>MPFTYSIEATRNLATTERCIQDIRNAPVRNRSTQFQLAQQNMLAYTFGEVIPGFASAGINGMDYRDVIGRPVENAVTEGTHFFRDDFRVDSNAKAKVAGDIFEIVSSAVMWNCAARWNSLMVGEGWRSQPRYSRPTLSPSPRRQVAVLNLPRSFDWVSLLVPESQEVIEEFRAGLRKDGLGLPTSTPDLAVVVLPEEFQNDEMWREEIAGLTRPNQILLSGAYQRLQGRVQPGEISLAVAFKRSLRSDRLYQPLYEANVMQLLLEGKLGAPKVEFEVHTLAPEGTNAFVTYEAASLYGLAEGRSAVHRAIRELYVPPTAADLARRFFAFLNERMELV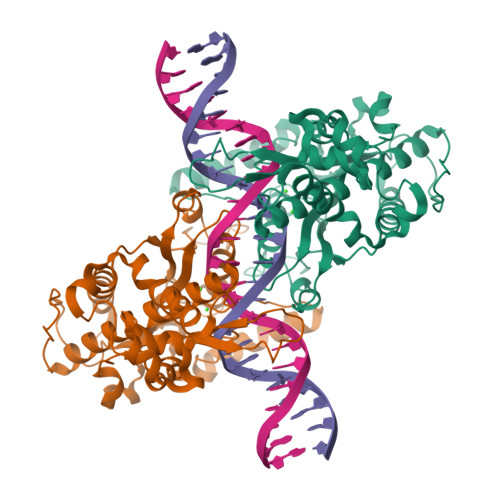NGENLYFQSHHHHHH[2x]> GAMNNHQIQELESNVDDLLHQLQLLK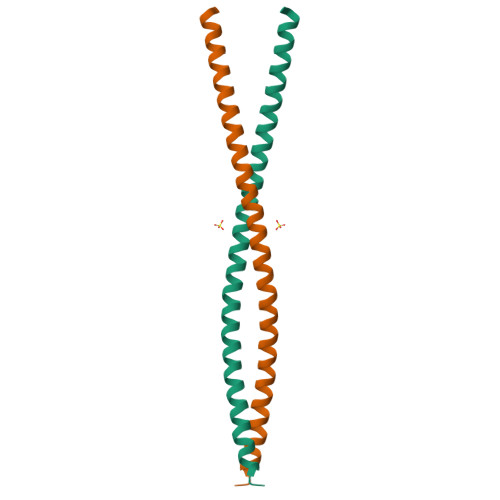EENNRKSMQISEMGKKISDLEVEKTAYRETLTNLNQELARLTNEEQSHRTEIFTLNASFKKQLNDIISQDNEKIEKLTG>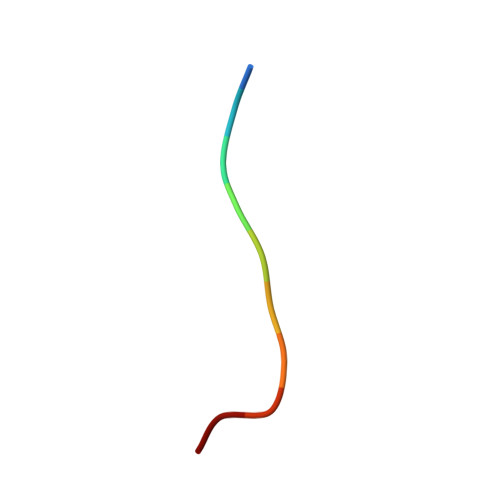 KGEADALSLD> MQVNRLPFFTNHFFDTYLLISEDTPVGSSVTQLLARDMDNDPLVFGVSGEEASRFFAVEPDTGVVWLRQPLDRETKSEFTVEFSVSDHQGVITRKVNIQ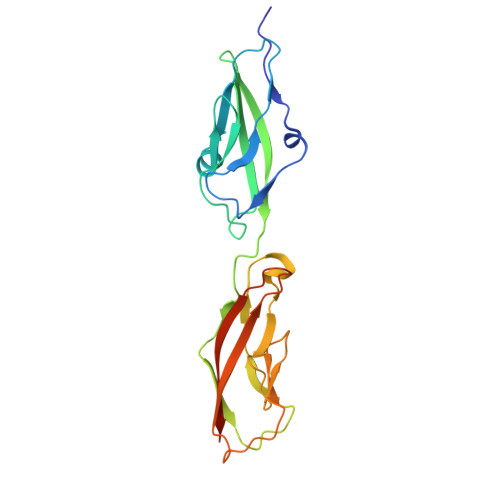VGDVNDNAPTFHNQPYSVRIPENTPVGTPIFIVNATDPDLGAGGSVLYSFQPPSPFFAIDSARGIVTVIQELDYEVTQAYQLTVNATDQDKTRPLSTLANLAIIITDLEHHHHHH53BP1 and TOPBP1 are multi-domain scaffold proteins that individually contribute to the genome stability functions of mammalian cells. Amongst other roles, TOPBP1 is involved in replication initiation through its interaction with TICCR/Treslin; the DNA damage checkpoint through interactions with 9-1-1, RHNO1/RHINO and ATR; and sister chromatid de-catenation and suppression of sister chromatid exchange via interactions with TOP2A and BLM. 53BP1 is recruited to sites of DNA damage through interaction with post-translationally modified histones and is strongly implicated in the process of choice between the non-homologous end joining and homologous recombination pathways of double-strand break (DSB) repair, as well as the localisation of activated ATM that is required for DSB repair in heterochromatin. Using a structurally-derived consensus pattern for phospho-ligand binding to the N-terminal regions of TOPBP1 and Rad4, we have now identified conserved phosphorylation sites in human 53BP1, and have biochemically and structurally characterised their interaction with BRCT domains of TOPBP1.

Of the four peptides, only the one centred on 53BP1-pThr670 bound tightly to TOPBP1-BRCT0,1,2 (Kd = 1.5 ± 0.2 μM). Treatment with λ-phosphatase eliminated binding, confirming that phosphorylation of the 53BP1 sequence is required. A high affinity interaction (Kd = 1.0 ± 0.2 μM) was still observed with TOPBP1-BRCT0,1,2-K155E, in which the phospho-binding site in the BRCT1 domain is mutationally disabled, but binding was ~10 fold weaker (Kd = 13.5 ± 6.2 μM) with TOPBP1-BRCT0,1,2-K250E, in which BRCT2 is mutated. These data implicate BRCT2 as the primary binding site, consistent with the presence of a hydrophilic residue −4 to the phosphothreonine, but with BRCT1 potentially providing a weaker alternative site. Co-crystallisation of TOPBP1-BRCT0,1,2 with the 53BP1-pThr670 phospho-peptide produced a crystal structure with peptide bound to BRCT2, consistent with the specificity it displays for that site in binding assays. The position and overall conformation of the bound peptide is similar to that previously described for the interaction of Crb2-derived phospho-peptides pThr187 and pThr235 bound to BRCT2 of Rad4. The phosphorylated side chain of 53BP1-Thr670 interacts with TOPBP1-Thr208 and TOPBP1-Lys250, which are topologically conserved in all BRCT domains capable of phospho-specific peptide interaction. The phosphate also interacts with the head group of TOPBP1-Arg215 which makes an additional hydrogen bond interaction with the side chain of 53BP1-Glu669. The side chain of the −3 residue of the phospho-peptide motif (see above), 53BP1-Ile667, packs into a hydrophobic pocket formed between the side chains of TOPBP1 residues Leu233, Gln249, Lys250 and Cys253. Additional specificity is provided by polar interactions between 53BP1-Glu669 and TOPBP1-Arg215, 53BP1-Glu666 and TOPBP1-Lys234, and 53BP1-Glu665 and the side chains of Arg256 and Trp257 of TOPBP1.

>GPMSRNDKEPFFVKFLKSSDNSKCFFKALESIKEFQSEEYLQIITEEEALKIKENDRSLYICDPFSGVVFDHLKKLGCRIVGPQVVIFCMHHQRCVPRAEHPVYNMVMSDVTISCTSLEKEKREEVHKYVQMMGGRVYRDLNVSVTHLIAGEVGSKKYLVAANLKKPILLPSWIKTLWEKSQEKKITRYTDINMEDFKCPIFLGCIICVTGLCGLDRKEVQQLTVKHGGQYMGQLKMNECTHLIVQEPKGQKYECAKRWNVHCVTTQWFFDSIEKGFCQDESIYKTEPRPEA[2x];> EVEEIPETPCESQGE>[2x]PSVYDAAAQLTADVKKDLRDSWKVIGSDKKGNGVALMTTLFADNQETIGYFKRLGDVSQGMANDKLRGHSITLMYALQNFIDQLDNPDDLVCVVEKLAVNHITRKISA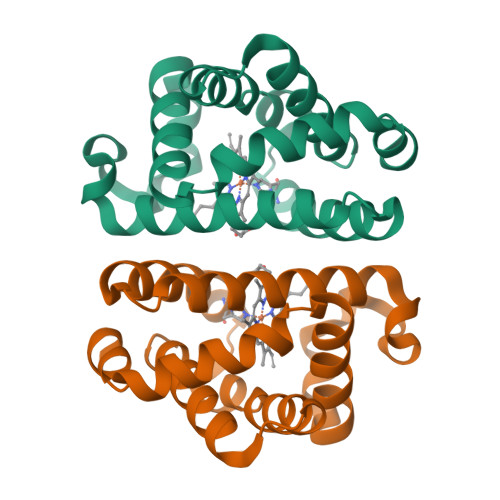AEFGKINGPIKKVLASKNFGDKYANAWAKLVAVVQAAL> MRSTQEERFEQRIAQETAIEPQDWMPDAYRKTLIRQIGQHAHSEIVGMLPEGNWITRAPTLRRKAILLAKVQDEAGHGLYLYSAAETLGCAREDIYQKMLDGRMKYSSIFNYPTLSWADIGVIGWLVDGAAIVNQVALCRTSYGPYARAMVKICKEESFHQRQGFEACMALAQG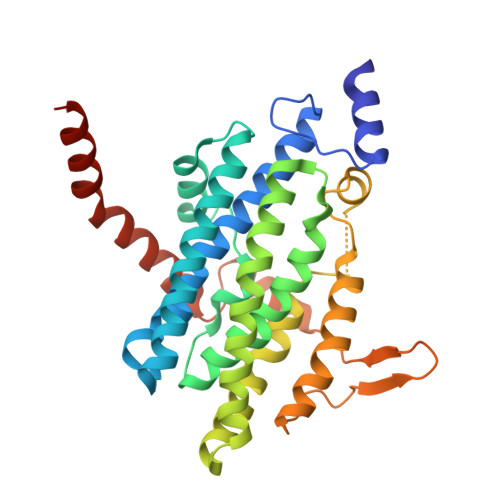SEAQKQMLQDAINRFWWPALMMFGPNDDNSPNSARSLTWKIKRFTNDELRQRFVDNTVPQVEMLGMTVPDPDLHFDTESGHYRFGEIDWQEFNEVINGRGICNQERLDAKRKAWEEGTWVREAALAHAQKQHARKVA>MEQETLEQVHLTEDGGVVKTILRKGEGGEENAPKKGN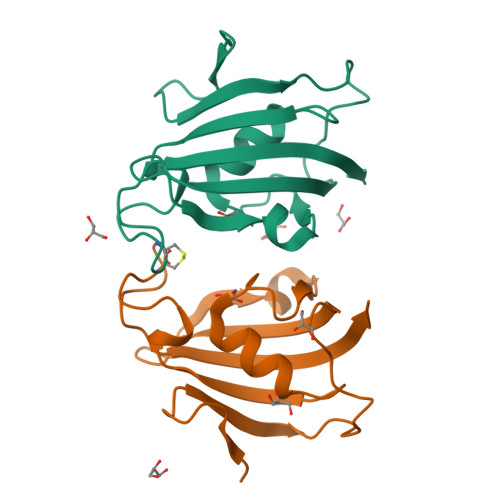EVTVHYVGKLESSGKVFDSSRERNVPFKFHLGQGEVIKGWDICVASMTKNEKCSVRLDSKYGYGEEGCGESIPGNSVLIFEIELISFRE[2x]>[4x]PEALQKWLQLTHEVEVQYYNIKKQNAEKQLMVAKEGAEKI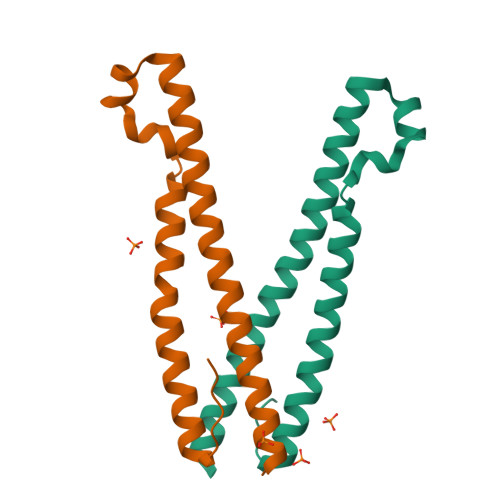KKKRNTLFGTFHVAHSSSLDDVDHKILTAKQALSEATAALRERLHRWQQIEILTGFQIVNN> MRRTRLVCTATPEKFSILGTTHPKPKRNGMGRN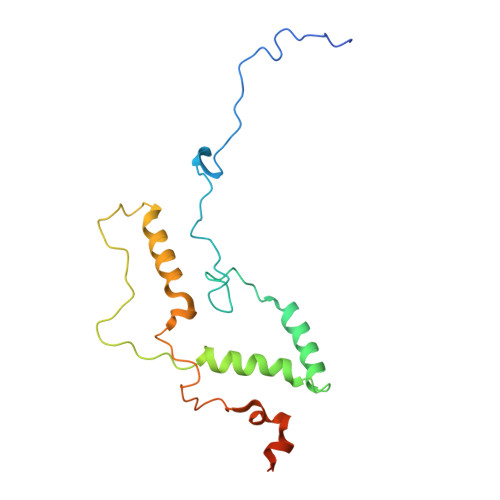NKMRSKPSDNVAWYDKGPVEWLPRPVRLTYDQLDQLRDWMMRETIAGRTEEFNKIRHLHREWSQHPLMPVLGDVEPKFPLNLYKQNHRAKRRFLVRWHKANSPTYWMWMPRGPAVATPLHRSSPSQFPEHWKSLARTSSSSSSSGSSSAAP>[14x]TVPDRDNDGIPDSLEVEGYTVD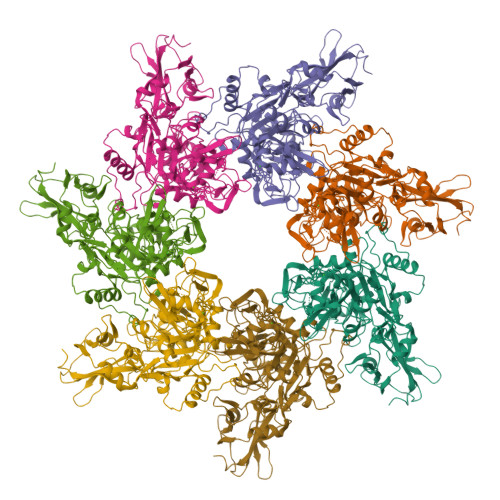VKNKRTFLSPWISNIHEKKGLTKYKSSPEKWSTASDPYSDFEKVTGRIDKNVSPEARHPLVAAYPIVHVDMENIILSKNEDQSTQNTDSQTRTISKNTSTSRTHTSEVHGNAEVHASFFDIGGSVSAGFSNSNSSTVAIDHSLSLAGERTWAETMGLNTADTARLNANIRYVNTGTAPIYNVLPTTSLVLGKNQTLATIKAKENQLSQILAPNNYYPSKNLAPIALNAQDDFSSTPITMNYNQFLELEKTKQLRLDTDQVYGNIATYNFENGRVRVDTGSNWSEVLPQIQETTARIIFNGKDLNLVERRIAAVNPSDPLETTKPDMTLKEALKIAFGFNEPNGNLQYQGKDITEFDFNFDQQTSQNIKNQLAELNATNIYTVLDKIKLNAKMNILIRDKRFHYDRNNIAVGADESVVKEAHREVINSSTEGLLLNIDKDIRKILSGYIVEIEDTEGLKEVINDRYDMLNISSLRQDGKTFIDFKKYNDKLPLYISNPNYKVNVYAVTKENTIINPSENGDTSTNGIKKILIFSKKGYEIG In this work, we engineer EUGO, a VAO-type oxidase, to catalyze the selective dehydrogenation of 4-n-propylguaiacol to isoeugenol. Similar to VAO, EUGO is active on various 4-substituted phenols and contains a covalently bound FAD. The oxidation of 4-alkylphenols starts with a hydride transfer from the Cα atom of the substrate to the N5 of the flavin cofactor. Consequently, a p-quinone methide is formed and stabilized in the active site. This reactive intermediate can subsequently be hydroxylated by the base-catalyzed attack of water, or tautomerise to the dehydrogenation product.

Interestingly, this additional mutation (D151E) resulted in a similar conversion compared to the parent mutant and similar steady-state kinetic parameters, but it displayed exquisite chemoselectivity by producing insignificant amounts of the undesired products. This prompted us to create the combined mutant D151E/S394V/Q425S-EUGO5X. As a result, the less constricted and tightly packed environment around the Cα atom of the substrate reduces the formation of the covalent adduct that impairs catalysis. The engineered D151E/S394V/Q425S-EUGO5X mutant was named 4-n-propylguaiacol oxidase (PROGO). The crystal structure of the D151E/S394V/Q425S-EUGO5X in a complex with 4-n-propylguaiacol was solved at 2.4 Å resolution. It showed that the bulkier E151 sidechain points towards the propenyl Cα atom of the substrate, potentially sequestering the reactive quinone methide and obstructing attack of water. The Q425S mutation renders the environment on top of the substrate less packed, creating a looser niche around the substrate side chain. This allows the 4-n-propylguaiacol to rotate slightly away from the flavin N5 as the substrate side chain can partly occupy the space vacated by removing the Q425 carboxamide group. Gratifyingly, this eightfold EUGO mutant was found to display all desired properties: conversion of 4-n-propylguaiacol led to the rapid formation of isoeugenol as the main product (97%). Characterization of the purified enzyme revealed that the kcat had improved by two orders of magnitude relative to wild-type EUGO, whilst retaining the thermostability of EUGO5X mutant. By introducing two more mutations (D151E and Q425S), a variant was created that combined all desired features (stability, selectivity and activity), acting as an efficient 4-n-propylguaiacol oxidase (PROGO).

>MTRTLPPGVSDERFDAALQRFRDVVGDKWVLSTADELEAFRDPYPVGAAEANLPSAVVSPESTEQVQDIVRIANEYGIPLHPVSTGKNNGYGGAAPRLSGSVIVKTGERMNRILEVNEKYGYALLEPGVTYFDLYEYLQSHDSGLMLDCPELGWGSVVGNTLDRGVGYTPYGDHFMWQTGLEVVLPQGEVMRTGMGALPGSDAWQLFPYGFGPFPDGMFTQSNLGIVTKMGIALMQRPPASQSFLITFDKEEDLEQIVDIMLPLRINMAPLQNVPVLRNIFMDAAAVSKRTEWFDGDGPMPAEAIERMKKDLDLGFWNFYGTLYGPPPLIEMYYGMIKEAFGKIPGARFFTHEERDDRGGHVLQDRHKINNGIPSLDELQLLDWVPNGGHIGFVPVSAPDGREAMKQFEMVRNRANEYNKDYMASFIIGLREMYHVCLFIYDTADPEAREEILQMTKVLVREAAEAGYGEYRTHNALMDDVMATFNWGDGALLKFHEKIKDALDPNGIIAPGKSGIWPQRFRGQNL[8x]> GDELYRQSLEIISRYLREQATGAKDTKPMGRSGATSRKALETLRRVGDGVQRNHETAFQGMLRKLDIKNEDDVKSLSRVMIHVFSDGVTNWGRIVTLISFGAFVAKHLKTINQESCIEPLAESITDVLVRTKRDWLVKQRGWDGFVEFFH;>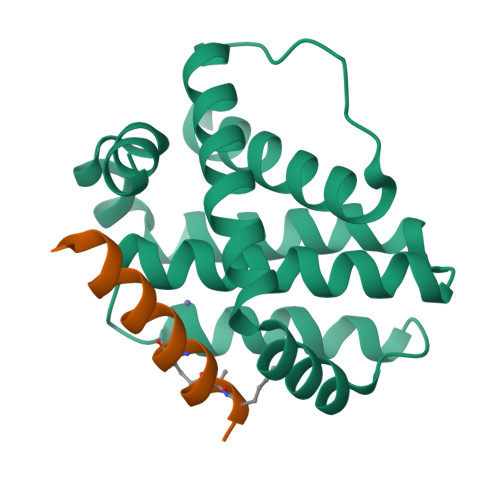 IWLLQSLLRLGDEINAYYARRX> MTVGTRRAAYATLITSDA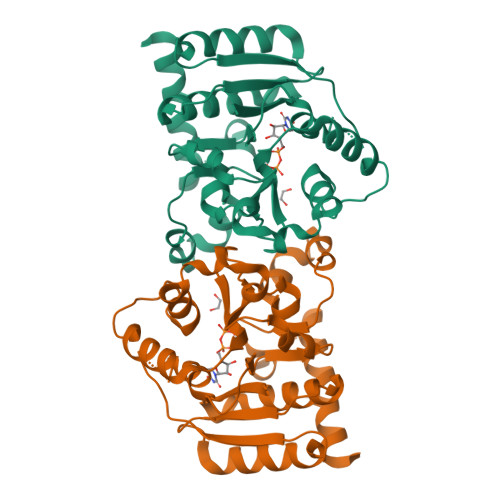YVMGVEALVYSLFKARVAFPLVVLHSSQVTQPTVAKLTRFCAPFQSSTWRISFRSVPDIGIPDEVTDRSTVHVPGWVNSGYTKLHIFAMDDFEQIVYIDADAIVLQNVDELFDRSTSFAAAPDVFPPDRFNAGVLVIRPNKQLFADLLAKAKELKSYDGGDTGFLNAFFPKWFESDAASRLPFGYNAQRTMYWLVNGKNPGYWNAVQPLKILHYSSNPKPWEDPSRKGDLEILWWQMYTESRCMSFLG> FNDNYSSTSTVYATSNEATDSRGSEHLRYPYLECIKIGMSRDYLENCVKVSFPTSQDMFYDAYPSTESDGAKTRTK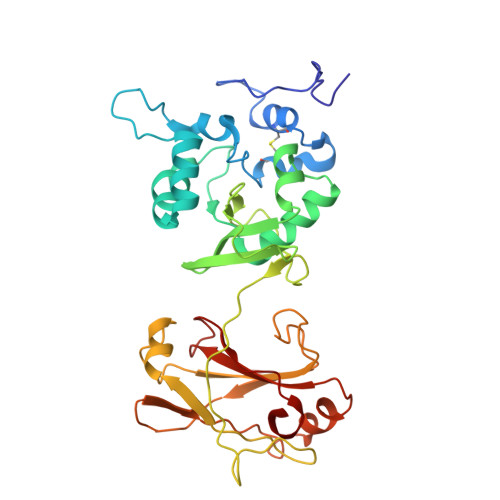EDFSARLLAGDYDSLQKLYIDFYLAQTTFDWEIPTRDQIETLVNYANEGKLSTALNQEYITGRFLTKENGRYDIVNVGGVPDNTPVKLPAIVSKRGLMGTTSVVNAIPNEIYPHIKVYEGTLSRLKPGGAMIAVLEYDVNELSKHGYTNLWDVQFKVLVGVPHAETGVIYDPVYEETVKPYQPSNNLTGKKLYNVSTNDMHNGYKWSNTMFSNSNYKTQILLTKGDGSGVKLYSKAYSENFK Central to ERQC is the ER-resident 170-kDa enzyme UDP-glucose:glycoprotein glucosyltransferase (UGGT). The enzyme selectively reglucosylates a misfolded glycoprotein on one of its N-glycans and promotes its association with the ER lectins calnexin and calreticulin, thus mediating its ER retention. The full-length Chaetomium thermophilum UGGT (CtUGGT) crystal structures revealed four DsbA-like domains (TRXL1–4) arranged in a long arc, terminating in two β sandwiches (βS1 and βS2) tightly clasping the glucosyltransferase family 24 (GT24) domain (Roversi et al., 2017). Overall, UGGT's motions can be described in simple terms as two rigid groups of domains moving with respect to one another.

To probe the functional role of the “clamping” motion uncovered in the present analysis, we engineered four double-cysteine CtUGGT mutants, CtUGGTG178C/A786C, CtUGGTG177C/A786C, CtUGGTG179C/T742C, and CtUGGTS180C/T742C, all designed to form disulfide bridges across the TRXL1 and TRXL3 domains, clamping shut the cleft between them. The presence of the engineered disulfide bridges in the remaining three mutants was confirmed by mass spectrometry. The crystal structures of CtUGGTG177C/A786C and CtUGGTS180C/T742C were determined to about 4.6-Å resolution. Both crystal structures show the TRXL3 domain tethered to the TRXL1 domain by the extra disulfide bridge. We tested the in vitro activity of the three “clamped-shut” double Cys mutants (in addition to the activity of the wild type and the already published CtUGGTD611C/G1050C) on urea-misfolded bovine thyroglobulin. As to the UGGT clamping motion, we tested two a priori rather similar double-cysteine mutants, CtUGGTS180C/T742C and CtUGGTG177C/A786C, both designed to clamp the TRXL1-TRXL3 domains shut. Surprisingly, the two mutants differ in their ability to reglucosylate urea-misfolded bovine thyroglobulin, with the former mutant more active than (and the latter mutant having similar activity to) wild-type CtUGGT. These observations point to the possibility that each misfolded glycoprotein substrate may depend to a different degree on a different subset of UGGT inter-domain conformational degrees of freedom.

> ETGQVAASPSINVALKAAFPSPPYLVELLETAASDNTTIYYSLLDRIAKGHFAEATTDKALYEKFLEVLRDDGHMDPEALSAFKLALSLRTATPRVEAHYQYYTATVEPSLSGTQEGCDQWFLIDGEQYCSPTLDTSHGKVKGEDQLRTLPFDRKFGVGCRDVILYADITSKSFAPFHEVAMDLAKKGKASYRVRYRRSPSHSRESLSVNGYGVELVLKRTDYIVIDDRDTGAAAKPAEENDQKPLVGHETVLDDGEEIADIKPLEKSELAALGMKAASFVMQSEKPFEALLKLTQDFPKYSNSLGSQNVSAEFEAEHRGNREVFLPEGSNVLWLNGLHLIDRQIQPFGLVDLLTRERKLIKSVLDLGLTGQQAVDLLGHAEVAHAKSGDDEPRRFDWRDDIEEGQVIIWLNNLEKDKRYKSFSPSIWVLIHHFGHGLPQIRRDVFNLVVPVDLTKADDVKIVVEGLLSFVKRLIPVRFGFVPLTPTGQAIDQAKVVYYLLENYGLAAATAYLEKSYEEQSTGQPNERIFNEVIKDKSLRPDGVELSFKDIFISEKHEKQIHLSKHWVERLRAGGDVPTVFFDGFPIPREDNWLRVMNHRLMQDLQALQQAGYFGMLNESMWLPGFFLEKALSRRNTLIFPEDKNELTVLNVNKIYIENHDLMSKVPVIEASKESTRDDWAALTVVADLDDIEGQELVYYALRFRKSNDGVRLDIVHNPKDCSRSPSVLAQRLKSREDKLLDFTRFLDLETALETGEFEPDVAYDASLANFLASSNMKAGDNFVILNGRVLGPITSADDFKKEDFEVFLQAERRTRILPVYKALEDLGLDDKVSGPLSAAKLTSVTALSTISDLPQGIFDNAPTVRTTLFKQWNSTYTSFEVGDASTATIFFVAVINPASEIGQRWVAVLKVLSELEGVHLRVFLNPTVMIEELPVKRFYRYVLSSSPSFDESGKVKALSARFTGVPRETLLVVGMDVPPAWLVTSKVAVDDLDNLRIKDIKAKRGTEHVEAIYELEHILIEGHSREIPGAHAPRGVQLVLETENNPHFADTIIMANLGYFQFKANPGVYNIRLKEGRSSEIFTLESVGAKGWGPIPGDDNTEVVLMDFQGTTLYPRLRRKPGMEEEDVLEPSTKSGEESGSGARNLVSRGIKFAEGLLGRGNKAAEATKSVSKTEHAEINIFSVASGHLYERMLNIMMASVMHHTNHTVKFWFIEQFLSPSFKDFIPHMAAEYGFKYEMVTYKWPHWLRQQKEKQREIWGYKILFLDVLFPLSLDKVIFVDADQIVRTDMYDLVEHPLDGAPYGFAPMCDSRVEMEGYRFWKTGYWANYLKGKPYHISALYVVDLQRFRELAAGDRLRQQYHALSADPNSLANLDQDLPNHMQFTIPIATLPQEWLWCETWCSDETLKDARTIDLCNNPMTKEPKLDRARRQVPEWTKYDEEIAELARRVREEKPKKKEEEKVQKNPKSRRLDGDEEEVKTVREGTKHHHHHH4-[2-AMINO-5-(1,3-BENZODIOXOL-4-YL)PYRIDIN-3-YL]BENZAMIDE | C19 H15 N3 O3 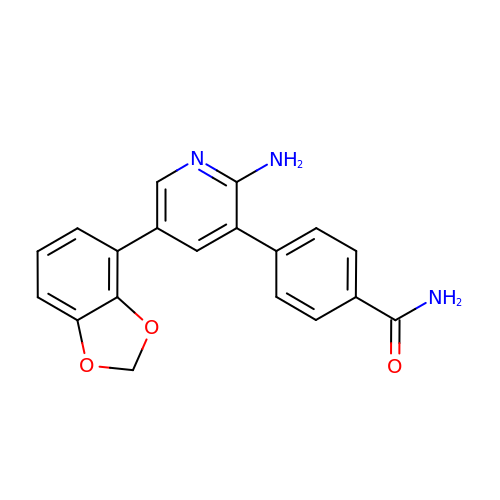| UBOGEBHIZSQBBD-UHFFFAOYSA-N>MGRSHHHHHHGSLVPRGSEQGSNVNHLIKVTDQSITEGYDDSDGIIKAHDAENLIYDVTFEVDDKVKSGDTMTVNIDKNTVPSDLTDSFAIPKIKDNSGEIIATGTYDNTNKQITYTFTDYVDKYENIKAHLKLTS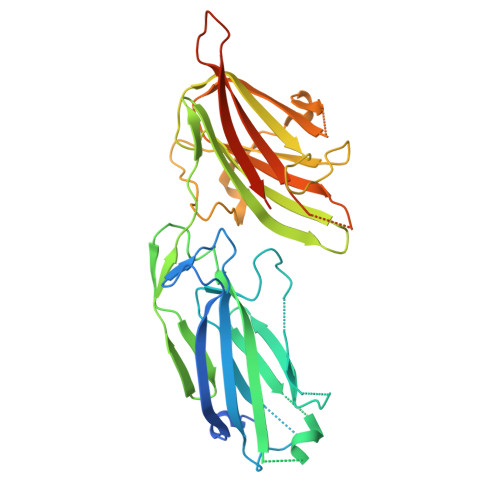YIDKSKVPNNNTKLDVEYKTALSSVNKTITVEYQKPNENRTANLQSMFTNIDTKNHTVEQTIYINPLRYSAKETNVNISGNGDEGSTIIDDSTIIKVYKVGDNQNLPDSNRIYDYSEYEDVTNDDYAQLGNNNDVNINFGNIDSPYIIKVISKYDPNKDDYTTIQQTVTMQTTINEYTGEFRTASYDNTIAFSTSSGQGQGDLPPEK[4x]> MGHHHHHHMPVVDSDGDAVQLNLGGNYPLYTIQSAAIGFRGGLSTLRKDACKSYVYEAPETDRGLPVGFSASATSQPVMQLGSRYKFSFSMPVPLICDTAWSIGKSETNGGISFQPITAGDYFYLNNFSWFEARSTEETGVYKLAACSCEFCKIACPEVGSFNVN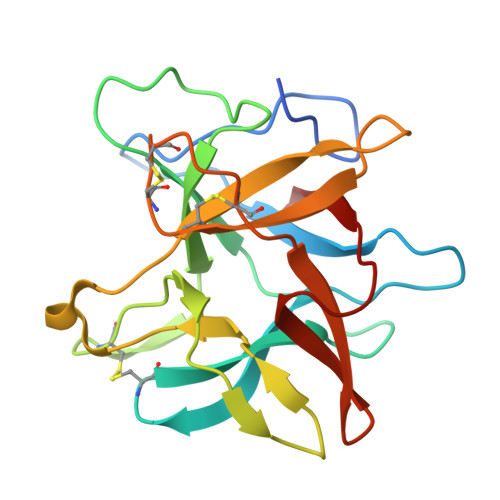GRTLLGIGGEHFTVQFQKFD(3S,5R,7R,8S,9S,10R)-7-(hydroxymethyl)-3-(2-naphthyl)-1,6-dioxa-2-azaspiro[4.5]decane-8,9,10-triol | C18 H21 N O6 | 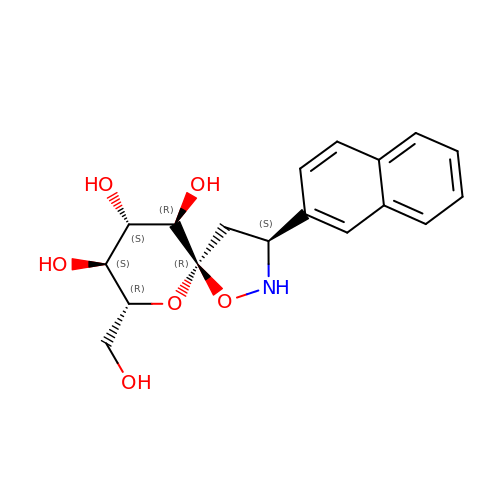ZCJBDRSKHARECB-PYTCMNEWSA-N Geranyl 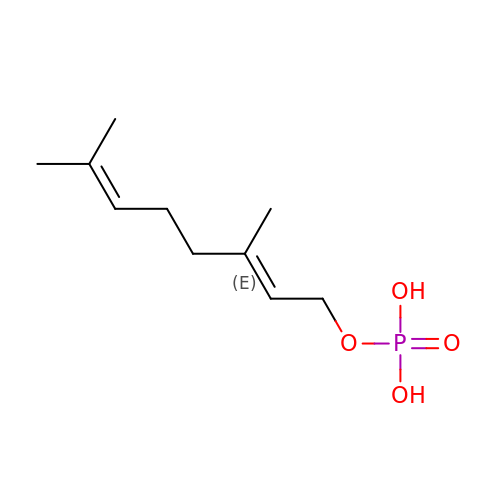phosphate | C10 H19 O4 P | FFOWJDCTFSWUMJ-JXMROGBWSA-N> VHFKDGVYENIPFKVKGRKTPYALS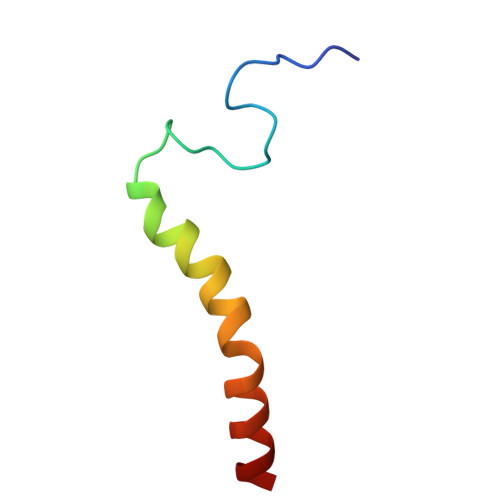HFGFFAIGFAVPFVACYVQLKK> GSADETLSQTKVLL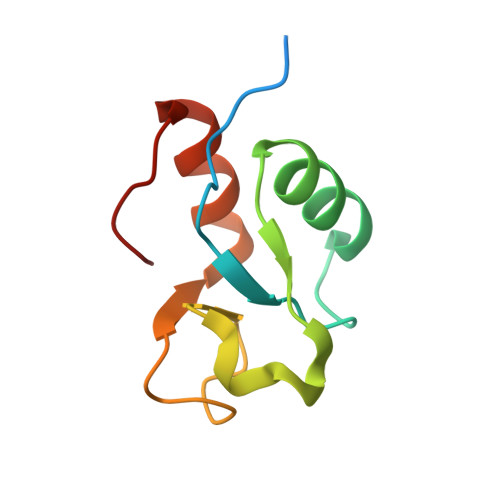DIFTGVRLYLPPSTPDFSRLRRYFVAFDGDLVQEFDMTSATHVLGSRDKNPAAQQVSPEWIWACIRKRRLVAPS>[2x]LPTSNPAQELEARQLGRTTRDDLINGNSASCADVIFIYARGSTETGNLGT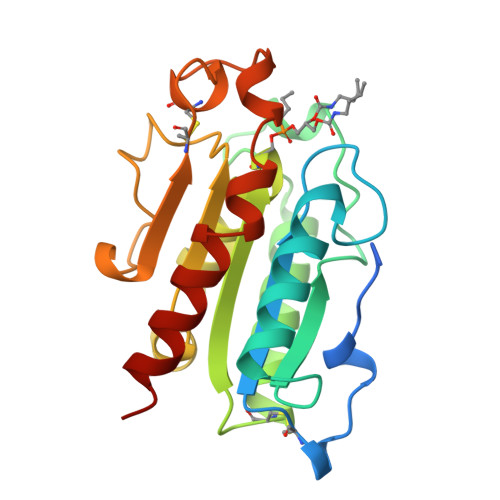LGPSIASNLESAFGKDGVWIQGVGGAYRATLGDNALPRGTSSAAIREMLGLFQQANTKCPDATLIAGGYSQGAALAAASIEDLDSAIRDKIAGTVLFGYTKNLQNRGRIPNYPADRTKVFCNTGDLVCTGSLIVAAPHLAYGPDARGPAPEFLIEKVRAVRGSA> MEVKYRGPSDDKLECEFLENNLLSCLREKSVQDNVAKMTCRPEFLVWFFL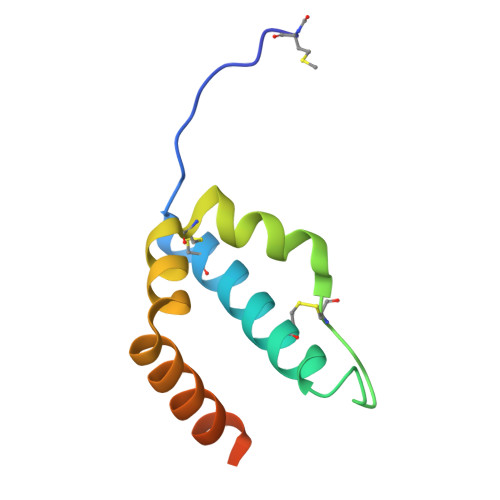ECPTKAAVYHDPKGLRNIFIQDKIKQKGSDDGVLSKDD> MAQILPIRFQEHLQLQNLGINPANIGFSTLTMESDKFICIREKVGEQAQVVIIDMNDPSNPIRRPISADSAIMNPASKVIALKAGKTLQIFNIEMKSKMKAHTMTDDVTFWKWISLNTVALVTDNAVYHWSM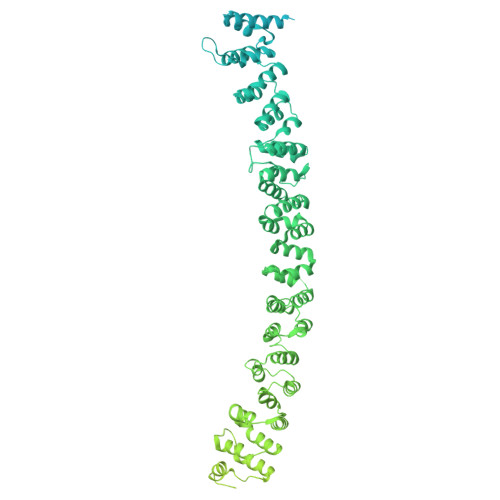EGESQPVKMFDRHSSLAGCQIINYRTDAKQKWLLLTGISAQQNRVVGAMQLYSVDRKVSQPIEGHAASFAQFKMEGNAEESTLFCFAVRGQAGGKLHIIEVGTPPTGNQPFPKKAVDVFFPPEAQNDFPVAMQISEKHDVVFLITKYGYIHLYDLETGTCIYMNRISGETIFVTAPHEATAGIIGVNRKGQVLSVCVEEENIIPYITNVLQNPDLALRMAVRNNLAGAEELFARKFNALFAQGNYSEAAKVAANAPKGILRTPDTIRRFQSVPAQPGQTSPLLQYFGILLDQGQLNKYESLELCRPVLQQGRKQLLEKWLKEDKLECSEELGDLVKSVDPTLALSVYLRANVPNKVIQCFAETGQVQKIVLYAKKVGYTPDWIFLLRNVMRISPDQGQQFAQMLVQDEEPLADITQIVDVFMEYNLIQQCTAFLLDALKNNRPSEGPLQTRLLEMNLMHAPQVADAILGNQMFTHYDRAHIAQLCEKAGLLQRALEHFTDLYDIKRAVVHTHLLNPEWLVNYFGSLSVEDSLECLRAMLSANIRQNLQICVQVASKYHEQLSTQSLIELFESFKSFEGLFYFLGSIVNFSQDPDVHFKYIQAACKTGQIKEVERICRESNCYDPERVKNFLKEAKLTDQLPLIIVCDRFDFVHDLVLYLYRNNLQKYIEIYVQKVNPSRLPVVIGGLLDVDCSEDVIKNLILVVRGQFSTDELVAEVEKRNRLKLLLPWLEARIHEGCTEPATHNALAKIYIDSNNNPERFLRENPYYDSRVVGKYCEKRDPHLACVAYERGQCDLELINVCNENSLFKSLSRYLVRRKDPELWGSVLLESNPYRRPLIDQVVQTALSETQDPEEVSVTVKAFMTADLPNELIELLEKIVLDNSVFSEHRNLQNLLILTAIKADRTRVMEYINRLDNYDAPDIANIAISNELFEEAFAIFRKFDVNTSAVQVLIEHIGNLDRAYEFAERCNEPAVWSQLAKAQLQKGMVKEAIDSYIKADDPSSYMEVVQAANTSGNWEELVKYLQMARKKARESYVETELIFALAKTNRLAELEEFINGPNNAHIQQVGDRCYDEKMYDAAKLLYNNVSNFGRLASTLVHLGEYQAAVDGARKANSTRTWKEVCFACVDGKEFRLAQMCGLHIVVHADELEELINYYQDRGYFEELITMLEAALGLERAHMGMFTELAILYSKFKPQKMREHLELFWSRVNIPKVLRAAEQAHLWAELVFLYDKYEEYDNAIITMMNHPTDAWKEGQFKDIITKVANVELYYRAIQFYLEFKPLLLNDLLMVLSPRLDHTRAVNYFSKVKQLPLVKPYLRSVQNHNNKSVNESLNNLFITEEDYQALRTSIDAYDNFDNISLAQRLEKHELIEFRRIAAYLFKGNNRWKQSVELCKKDSLYKDAMQYASESKDTELAEELLQWFLQEEKRECFGACLFTCYDLLRPDVVLETAWRHNIMDFAMPYFIQVMKEYLTKVDKLDASESLRKEEEQATETQ>MAPTFQTALFFTIISLSFAAPNAKQVRWCAISDLEQKKCNDLVGSCNVPDITLVCVLRSSTEDCMTAIKDGQADAMFLDSGEVYEASKDPYNLKPIIAEPYSSNRDLQKCLKERQQALAKKMIGHYIPQCDEKGNYQPQQCHGSTGHCWCVNAMGEKISGTNTPPGQTRATCERHELPKCLKERQVALGGDEKVLGRFVPQCDEKGNYEPQQFHGSTGYSWCVNAIGEEIAGTKTPPGKIPATCQKHDLVTTCHYAVAMVKKSSAFQFNQLKGKRSCHSGVSKTDGWKALVTVLVEKKLLSWDGPAKESIQRAMSKFFSVSCIPGATQTNLCKQCKGEEGKNCKNSHDEPYYGNYGAFRCLKEDMGDVAFLRSTALSDEHSEVYELLCPDNTRKPLNKYKECNLGTVPAGTVVTRKISDKTEDINNFLMEAQKRQCKLFSSAHGKDLMFDDSTLQLALLSSEVDAFLYLGVKLFHAMKALTGDAHLPSKNKVRWCTINKLEKMKCDDWSAVSGGAIACTEASCPKGCVKQILKGEADAVKLEVQYMYEALMCGLLPAVEEYHNKDDFGPCKTPGSPITDFGTLRAVALVKKSNKDINWNNIKGKKSCHTGVGDIAGWVIPVSLIRRQNDNSDIDSFFGESCAPGSDTKSNLCKLCIGDPKNSAANTKCSLSDKEAYYGNQGAFRCLVEKGDVAFVPHTVVFENTDGKNPAVWAKNLKSEDFELLCLDGSRAPVSNYKSCKLSGIPPPAIVTREESISDVVRIVANQ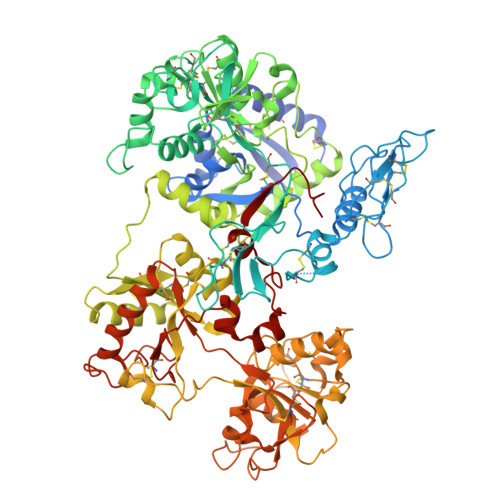QSLYGRKGFEKDMFQLFSSNKGNNLLFNDNTQCLITFDRQPKDIMEDYFGKPYYTTVYGASRSAMSSELISACTIKHCSNSLEVL[2x]>[2x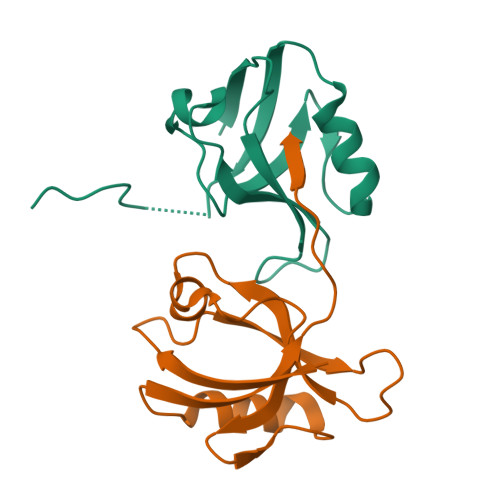]GSHMPQPELQLIKLHKNSNGMGLSIVAAKGAGQEKLGIYIKSVVPGGAADADGRLQAGDQLLRVDGQSLIGITQERAADYLVRTGPVVSLEVAKQGAIIREIIV> ETTSSIGEKVWDDKDNQDGKRPEKVSVNLLANGEKVKTLDVTSETNWKYEFKDLPKYDEGKKIEYTVTEDHVKDYTTDINGTTI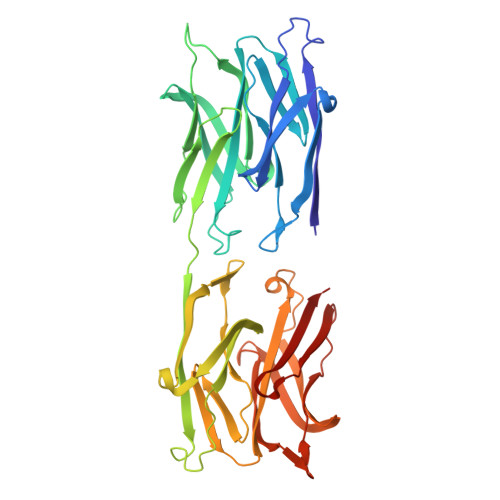TNKYTPGETSATVTKNWDDNNNQDGKRPTEIKVELYQDGKATGKTAILNESNNWTHTWTGLDEKAKGQQVKYTVEELTKVKGYTTHVDNNDMGNLITTNKYTPETTSSIGEKVWDDKDNQDGKRPEKVSVNLLANGEKVKTLDVTSETNWKYEFKDLPKYDEGKKIEYTVTEDHVKDYTTDINGTTITNKYTPGETSATVTKNWDDNNNQDGKRPTEIKVELYQDGKATGKTAILNESNNWTHTWTGLDEKAKGQQVKYTVEELTKVKGYTTHVDNNDMGNLITTNKYT>MCGRFLRRLLAEESRRSTPVGRLLLPVLLGFRLVLLAASGPGVYGDEQSEFVCHTQQPGCKAACFDAFHPLSPLRFWVFQVILVAVPSALYMGFTLYHVIWHWELSGKGKEEETLIQGREGNTDVPGAGSLRLLWAYVAQLGARLVLEGAALGLQYHLYGFQMPSSFACRREPCLGSITCNLSRPSEKTIFLKTMFGVSGFCLLFTFLELVLLGLGRWWRTWKHKSSSSKYFLTSESTRRHKKATDSLPVVETKEQFQEAVPGRSLAQEK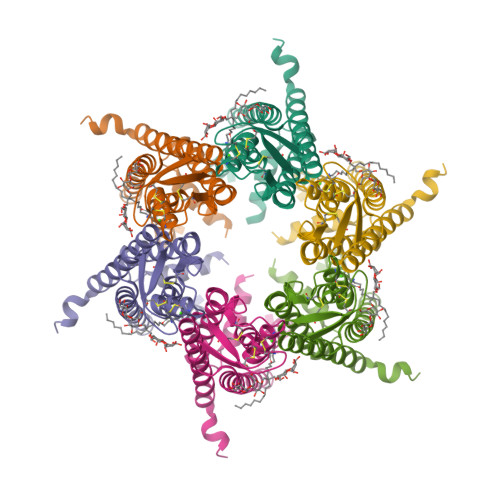QRPVGPRDA[6x]(4-phenylpiperazin-1-yl)(1H-1,2,3-triazol-1-yl)methanone | C13 H15 N5 O | 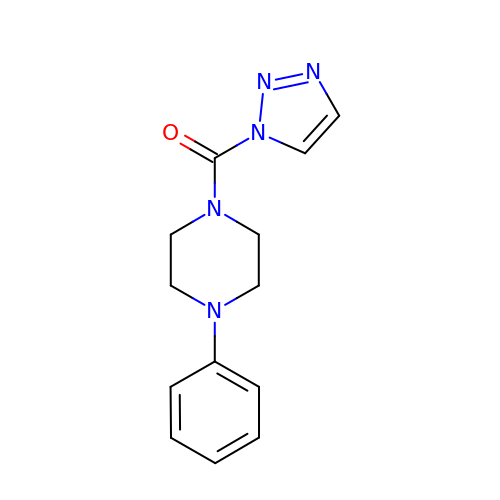ILKSIXGCKDCMDG-UHFFFAOYSA-N> QENRLLNESESSSQGLLGYYFSDLNFQAPMVVTSSTTGDLSIPSSELENIPSENQYFQSAIWSGFIKVKKSDEYTFATSADNHVTMWVDDQEVINKASN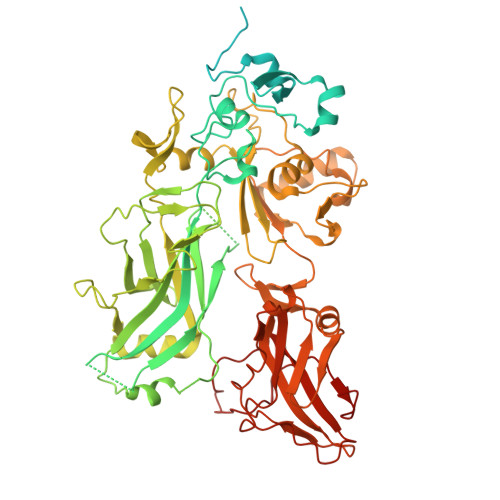SNKIRLEKGRLYQIKIQYQREDPTEKGLDFKLYWTDSQNKKEVISSDNLQLPELKQKSSNSLEVLFQGSTSAGPTVPDRDNDGIPDSLEVEGYTVDVKNKRTFLSPWISNIHEKKGLTKYKSSPEKWSTASDPYSDFEKVTGRIDGNVSPEANHPLVAAYPIVHVDMENIILSKNEDQSTQNTDSQTRTISKNTSTSRTHTSEVHGNAEVHASFFDIGGSVSAGFSNSNSSTVAIDHSLSLAGERTWAETMGLNTADTARLNANIRYVNTGTAPIYNVLPTTSLVLGKNQTLATIKAKENQLSQILAPNNYYPSKNLAPIALNAQDDFSSTPITMNYNQFLELEKTKQLRLDTDQVYGNIATYNFENGRVRVDTGSNWSEVLPQIQETTARIIFNGKDLNLVERRIAAVNPSDPLETTKPDMTLKEALKIAFGFNEPNGNLQYQGKDITEFDFNFDQQTSQNIKNQLAELNATNIYTVLDKIKLNAKMNILIRDKRFHYDRNNIAVGADESVVKEAHREVINSSTEGLLLNIDKDIRKILSGYIVEIEDTEGLKEVINDRYDMLNISSLRQDGKTFIDFKKYNDKLPLYISNPNYKVNVYAVTKENTIINPSENGDTSTNGIKKILIFSKKGYEIG> MTPMKTYDLIVIGTGPGGYHAAIRAAQLGLKVLAVEAGEVGGVCLNVGCIPTKALLHAAETLHHLKVAEGFGLKAKPELDLKKLGGWRDQVVKKLTGGVGTLLKGNGVELLRGFARLVGPKEVEVGGERYGAKSLILATGSEPLELKGFPFGEDVWDSTRALKVEEGLPKRLLVIGGGAVGLELGQVYRRLGAEVTLIEYMPEILPQGDPETAALLRRALEKEGIRVRTKTKAVGYEKKKDGLHVRLEPAEGGEGEEVVVDKVLVAVGRKPRTEGLGLEKAGVKVDERGFIRVNARMETSVPGVYAIGDAARPPLLAHKAMREGLIAAENAAGKDSAFDYQVPSVVYTSPEWAGVGLTEEEAKRAGYKVKVGKFPLAASGRALTLGGAEGMVKVVGDEETDLLLGVFIVGPQAGELIAE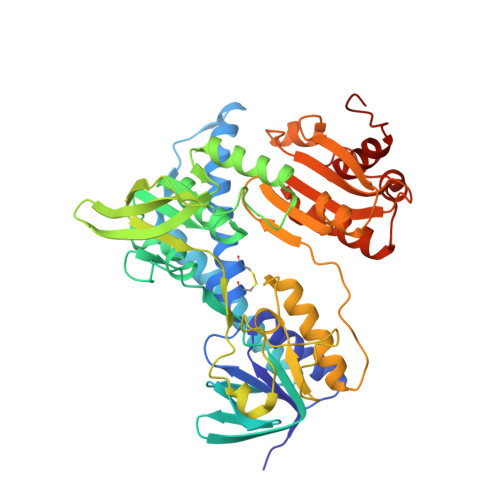AALALEMGATLTDLALTVHPHPTLSESLMEAAEAFHKQAIHILNR>MTVGNDDNLDKEIGQLLMCGFDGLEPTPGIIDLIENHNLGSIILFSRNIATPKQVQKLTHSLQQIARNAGHKRPLFIAVDQENGVVRRLGDSGTYLPGNMALGALGSSTAARNVAMAISKELLTLGMNWNLAPVLDVNNNPLNPVIGVRSYGQDPELVARMGLAQVEGYQRGKVATSIKHFPGHGDTATDSHLDVPVINKTLEELDKTELVPFKKALEAGGIACPTSVMVGHMLLPHFNKDVVSSIAPEIVRDLLRRRFGYKGVIITDCLEMDAVKETVGTPKGALMALQAGNDMAMISHTLAFQKDAFKVLYSALQEGQLDKDEIRQSLQRVAQLKDQFLNWDDVLQQADLKTMGSEAHATLSKELYDRVPTVVTNRKNTLPIRPAQTDKILFLAAHVPQTLAVDSEKEPFNSFHASLLKRHTNLEYIIYNEETPDLSQKIQEADWVIIGTANANLYPFQVRMVQQAQKLAKRLVVAAVMNPYDQMCFPQVDTYLVTYEYTPPAHEAAVRLIFGEIET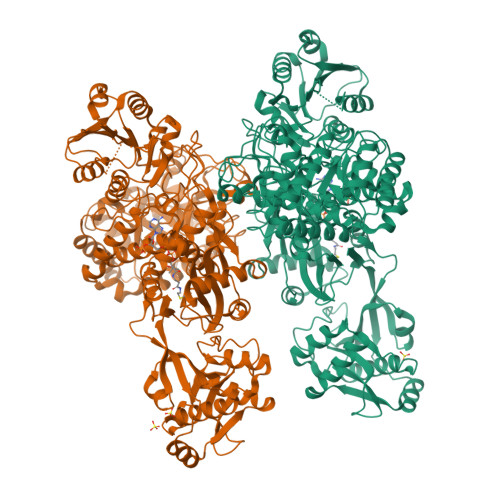RSRLPISIPNVDDAIAPATFIVDDYRNDDDLDHVTAMWDDIFGKDWPLRKDKINLGLQRAKLQKHKVARDSQGKIVGFVATQIVVVDNKKHGQLMLLMVSPSYQGKGVGTLLHDAALEHFREQGADCIKLGSTYPRFFPGVPDDDAQSRKAQAFFSKKGWRMDDNLVHDLIGDLQDYKVPDKIQARMLKEKIWFGRIKPSETWELYAFQQRNFPHWLSTYQHHVELGDYQDLIVARQDDENGRVIASLILNTTHVSHEYRSDLIWTDDKLFGERSGGMACVGVAQEERGRGIGIGIVAHANWLLKQRGVTKSYVDWVELLDFYSRVGYKTWRSYRLGHF[2x]> ATIKDV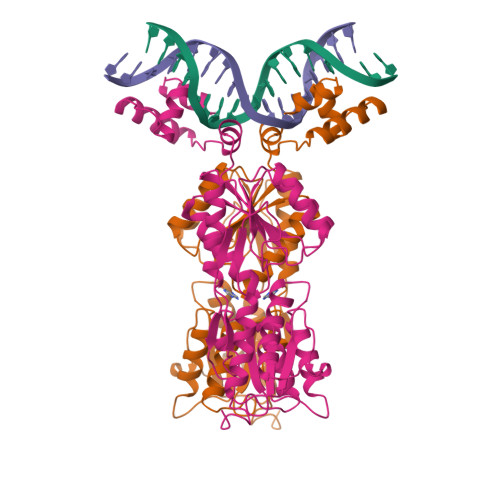AKRANVSTTTVSHVINKTRFVAEETRNAVWAAIKELHYSPSAVARSLAVNHTKSIGLLATSSEAAYFAEIIEAVEKNCFQKGYTLILGNAWNNLEKQRAYLSMMAQKRVDGLLVMCSEYPEPLLAMLEEYRHIPMVVMDWGEAKADFTDAVIDNAFEGGYMAGRYLIERGHREIGVIPGPLERNTGAGRLAGFMKAMEEAMIKVPESWIVQGDFEPESGYRAMQQILSQPHRPTAVFCGGDIMAMGALCAADEMGLRVPQDVSLIGYDNVRNARYFTPALTTIHQPKDSLGETAFNMLLDRIVNKREEPQSIEVHPRLIERRSVADGPFRDYRR> AQSVPYGVSQIKAPALHSQGYCGSNVKVAVIDSGIDSSHPDLKVAGGASFVPSETNPFQDNNSHGTHVAGTVAALNNSIGVLGVAPCASLYAVKVLGADGSGQYSWIINGIEWAIANNMDVINMSLGGPSGSAALKAAVDKAVASGVVVVAAAGN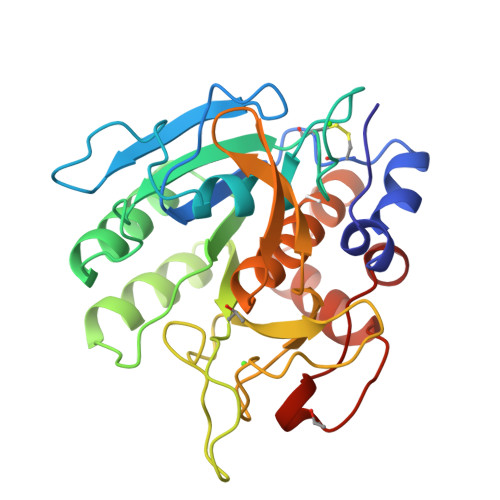EGTSGSSSTVGYPAKYPSVIAVGAVDSSNQRASFSSVGPELDVMAPGVSICSTLPGNKYGAKSGTSMASPHVAGAAALILSKHPNWTNTQVRSSLENTTTKLGDSFYYGKGLINVQAAAQ Acetylated lysine (Kac) in the N-terminal tail of H3 or H4 provides a binding scaffold for reader proteins such as those containing a bromodomain or Yaf9, ENL, AF9, Taf14, and Sas5 (YEATS) domain. Another Kac-binding domain, the YEATS domain, consists of approximately 130 residues and forms an antiparallel β-sheet structure that can recognize and bind Kac and some acylated lysines. In humans, four YEATS domains are present in four different proteins (AF9, ENL, YEATS2, and GAS41). Human YEATS domains bind to the acetylated N-terminal tail of histone H3; however, their Kac-binding preferences at the level of the nucleosome are unknown.

We determined the crystal structures of AF9-YEATS complexed with the K5/K8- (1.95 Å resolution) and K8/K12- (2.00 Å resolution) diacetylated H4 peptides. The crystal forms of AF9-YEATS in complex with K5/K8- and K8/K12-diacetylated peptides both belonged to the space group P1, and each asymmetric unit contained two AF9-YEATS molecules (molecules A and B). Molecule A in complex with the H4K5ac/K8ac peptide (chain A) and molecules A and B in complex with two H4K8ac/K12ac peptides (chains A and B) recognized H4K8ac at the aromatic cage. Molecule B in the H4K5ac/K8ac peptide complex did not bind the peptide at the aromatic cage because the aromatic cage was closed by conformational changes around Y78 in AF9. The electron density of H4K5ac was detected in the H4K5ac/K8ac peptide complex structure, but the position of the side chain of unmodified H4K5 in the H4K8ac/K12ac peptide complex could not be determined because of low electron density. K5ac and K12ac were located outside the aromatic cage; Nε of H4K5ac hydrogen bonded with E57 (left) and the added acetyl group of H4K12ac hydrogen bonded with D103 via a water molecule (right). Outside this cage, the main chain of unmodified H4K12 in the H4K5ac/K8ac peptide complex also hydrogen bonded with D103 via two water molecules, whereas its side chain was oriented toward the solvent (left). The interaction modes of AF9-YEATS with H4K8ac and with H3K9ac were the same: the aromatic cage of AF9-YEATS hydrophobically interacted with the aromatic residues F28, H56, F59, Y78, and F81; and the amide and the carbonyl oxygen of the Kac side chain formed hydrogen bonds with the hydroxyl group of S58 and the backbone amide of Y78. On the other hand, the increase of K1/2 toward K8/K12-diacetylated NCPs was 1.3-fold, which is the lowest among the three multiacetylated NCPs. This result suggests that the E57 residue is important for the interaction with multiacetylated NCPs containing H4K5ac.

>GSSGSSGMASSCAVQVKLELGHRAQVRKKPTVEGFTHDWMVFVRGPEHSNIQHFVEKVVFHLHESFPRPKRVCKDPPYKVEESGYAGFILPIEVYFKNKEEPRKVRFDYDLFLHLEGHPPVNHLRCEKLTFNNPTEDFRRKLLKA[2x];> SGRGKGGKGLGK> MDYKDDDDKGTMPSGFQQIGSEDGEPPQQRVTGTLVLAVFSAVLGSLQFGYNIGVINAPQKVIEQSYNETWLGRQGPEGPSSIPPGTLTTLWALSVAIFSVGGMISSFLIGIISQWLGRKRAMLVNNVLAVLGGSLMGLAN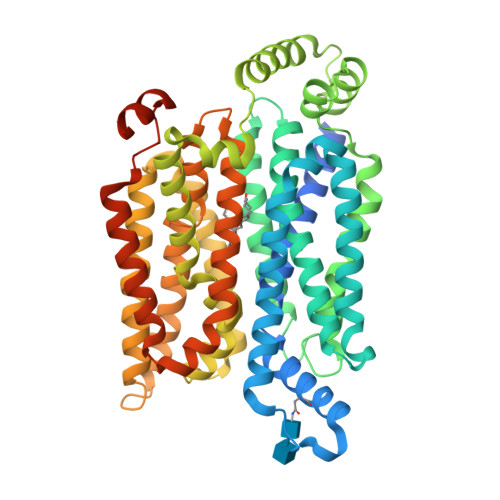AAASYEMLILGRFLIGAYSGLTSGLVPMYVGEIAPTHLRGALGTLNQLAIVIGILIAQVLGLESLLGTASLWPLLLGLTVLPALLQLVLLPFCPESPRYLYIIQNLEGPARKSLKRLTGWADVSGVLAELKDEKRKLERERPLSLLQLLGSRTHRQPLIIAVVLQLSQQLSGINAVFYYSTSIFETAGVGQPAYATIGAGVVNTVFTLVSVLLVERAGRRTLHLLGLAGMCGCAILMTVALLLLERVPAMSYVSIVAIFGFVAFFEIGPGPIPWFIVAELFSQGPRPAAMAVAGFSNWTSNFIIGMGFQYVAEAMGPYVFLLFAVLLLGFFIFTFLRVPETRGRTFDQISAAFHRTPSLLEQEVKPSTELEYLGPDEND> MSAYATQGFNLDDRGRRIVVDPVTRIEGHMRCEVNVDANNVIRNAVSTGTMWRGLEVILKGRDPRDAWAFVERICGVCTGCHALASVRAVENALDIRIPKNAHLIREIMAKTLQVHDHAVHFYHLHALDWVDVMSALKADPKRTSELQQLVSPAHPLSSAGYFRDIQNRLKRFVESGQLGPFMNGYWGSKAYVLPPEANLMAVTHYLEALDLQKEWVKIHTIFGGKNPHPNYLVGGVPCAINLDGIGAASAPVNMERLSFVKARIDEIIEFNKNVYVPDVLAIGTLYKQAGWLYGGGLAATNVLDYGEYPNVAYNKSTDQLPGGAILNGNWDEVFPVDPRDSQQVQEFVSHSWYKYADESVGLHPWDGVTEPNYVLGANTKGTRTRIEQIDESAKYSWIKSPRWRGHAMEVGPLSRYILAYAHARSGNKYAERPKEQLEYSAQMINSAIPKALGLPETQYTLKQLLPSTIGRTLARALESQYCGEMMHSDWHDLVANIRAGDTATANVDKWDPATWPLQAKGVGTVAAPRGALGHWIRIKDGRIENYQCVVPTTWNGSPRDYKGQIGAFEASLMNTPMVNPEQPVEILRTLHSFDPCLACSTH;> METKPRTPVLWLHGLECTCCSESFIRSAHPLAKDVVLSMISLDYDDTLMAAAGHQAEAILEEIMTKYKGNYILAVEGNPPLNQDGMSCIIGGRPFIEQLKYVAKDAKAIISWGSCASWGGVQAAKPNPTQATPVHKVITDKPIIKVPGCPPIAEVMTGVITYMLTFDRIPELDRQGRPKMFYSQRIHDKCYRRPHFDAGQFVEEWDDESARKGFCLYKMGCKGPTTYNACSTTRWNEGTSFPIQSGHGCIGCSEDGFWDKGSFYDRLTGISQFGVEANADKIGGTASVVVGAAVTAHAAASAIKRASKKNETSGSEHRSAWSHPQFEK

A prominent member of these so-called Knallgas bacteria is Cupriavidus necator H16 (formerly Ralstonia eutropha H16), which employs four different O2-tolerant [NiFe]-hydrogenases for generating cellular energy from the controlled oxidation of H2 in the presence of O2.5 Among them, only the tripartite membrane-bound [NiFe]-hydrogenase (MBH) is directly linked to the respiratory chain. The MBH large subunit contains the catalytic center composed of a nickel and an iron ion, which are coordinated to the protein by four Cys-derived thiolates. The most distal cluster relative to the active site is a [4Fe–4S] cluster coordinated by three cysteines and a histidine, while the medial cluster is a [3Fe–4S] species with three cysteines as protein anchors. However, in the proximal position, instead of a standard Cys4[4Fe–4S] cluster, the O2-tolerant MBHs possess a [4Fe–3S] cluster coordinated by six cysteine residues (Fig. 1 and S1†).13–16 The unique architecture of the [4Fe–3S] cluster is associated with a redox-dependent structural flexibility that allows two redox-transitions within a physiological potential region, i.e., the cofactor can assume a super-oxidized, an oxidized, and a reduced state. In order to obtain insight into the individual role of the supernumerary cysteines in the coordination and function of the [4Fe–3S] cluster, we purified C. necator MBH derivatives carrying exchanges of cysteine for glycine at the positions 19 and/or 120 in the small subunit HoxK, which are hereafter referred to as MBHC19G, MBHC120G and MBHC19G/C120G.

The electron density distribution was interpreted with 50% of Fe4 residing in a comparable position as in H2-reduced MBHC120G. However, an Fe4–S3 distance of 2.9 Å indicates the absence of a covalent bond. The remaining 50% of Fe4′ in oxidized MBHC120G were shifted by 1.2 Å to form a covalent bond with the backbone nitrogen of Cys20, bringing Fe4′ into hydrogen bonding distance (2.8 Å) with Glu76 of the MBH small subunit. This particular Fe4′ position differs by 0.6 Å from the classical Fe4 position of native MBH in the super-oxidized state, and the distance between Fe4′ and Sγ-Cys19 and Sγ-Cys20 is 2.9 Å and 2.7 Å, respectively. As observed for all single cluster variants of MBH, the Fe3 was found in a double conformation. Approximately 75% resided in the native Fe3 position and formed a covalent bond to S4 (Fe3–S4 distance 2.4 Å), consistent with the S4 occupancy. The remaining 25% of the Fe3 were shifted by 1.1 Å toward a more cubic conformation (Fe3′). However, a covalent binding to Sγ-Cys19 was not established (Fe3′ – Sγ-Cys19 distance 3.2 Å), resulting in a three-fold ligation of Fe3′ (Fig. S3b†). The proximal Cys5[4Fe–4S] cluster in oxidized MBHC120G is even more flexible, forming a new cluster scaffold with altered redox properties and electronic structure.5-[[3-[3-(dimethylamino)-1,2,4-oxadiazol-5-yl]-2-oxidanyl-phenyl]methylamino]-2~{H}-indazole-3-carboxylic acid | C19 H18 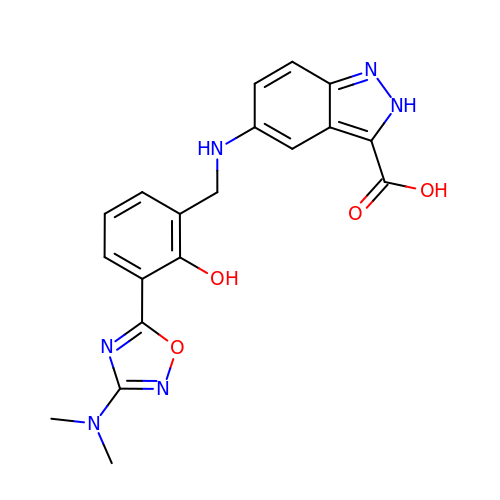N6 O4 | QZFNTDYKERMDQJ-UHFFFAOYSA-N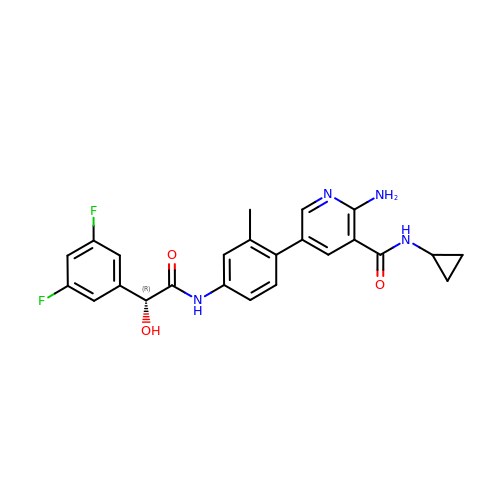2-amino-N-cyclopropyl-5-(4-{[(2R)-2-(3,5-difluorophenyl)-2-hydroxyacetyl]amino}-2-methylphenyl)pyridine-3-carboxamide | C24 H22 F2 N4 O3 | ZAEWPVUVQVUGEE-OAQYLSRUSA-N>MSLIASIGELLIDLISVEEGDLKDVRLFEKHPGGAPANVAVGVSRLGVKSSLISKVGNDPFGEYLIEELSKENVDTRGIVKDEKKHTGIVFVQLKGASPSFLLYDDVAYFNMT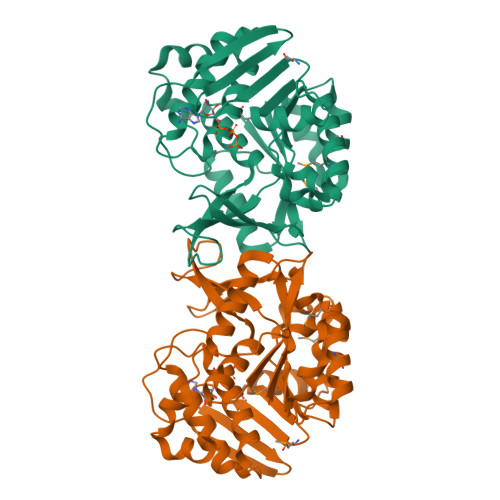LNDINWDIVEEAKIVNFGSVILARNPSRETVMKVIKKIKGSSLIAFDVNLRLDLWRGQEEEMIKVLEESIKLADIVKASEEEVLYLENQGVEVKGSMLTAITLGPKGFRLIKNETVVDVPSYNVNPLDTTGAGDAFMAALLVGILKLKGLDLLKLGKFANLVAALSTQKRGAWSTPRKDELLKYKEAREVLAEGHHHHHH[4x]The crystal structures and inhibitor complexes of two industrially important ω-aminotransferase enzymes from Pseudomonas aeruginosa and Chromobacterium violaceum have been determined in order to understand the differences in their substrate specificity. The two enzymes share 30% sequence identity and use the same amino acceptor, pyruvate; however, the Pseudomonas enzyme shows activity towards the amino donor β-alanine, whilst the Chromobacterium enzyme does not. Both enzymes show activity towards S-α-methylbenzylamine (MBA), with the Chromobacterium enzyme having a broader substrate range. It appears that the different rigidity of the protein scaffold contributes to the substrate specificity observed for the two ω-­aminotransferases.

We also present the crystal structure of C. violaceum Am:PyAT in complex with the inhibitor gabaculine. In comparison, the crystal structure of the C. violaceum gabaculine complex shows significant structural rearrangements from the structures of both the apo and holo forms of the enzyme. The C. violaceum Am:PyAT–mCPP complex was refined with partial occupancies of 0.7 and 0.6 in subunits A and B, respectively. The loop CV Ala57–Cys61 in chain A of the C. violaceum Am:PyAT–mCPP complex was built in two alternative conformations. The major conformation of this loop in chain A (occupancy of 0.7) folds differently, with the positions of CV Leu59 and CV Trp60 inverted at the bottom of the substrate pocket. The mCPP aromatic ring is rotated by approximately 15° between the two subunits of the C. violaceum Am:PyAT–mCPP complex. The carboxyl group of gabaculine forms a salt bridge with the side chain of CV Arg416 in the C. violaceum enzyme structure. The aromatic ring of mCPP is positioned in a hydrophobic pocket formed by residues CV Trp60, CV Tyr153, CV Ala231, CV Ile262, CV Leu59 and CV His318 from the adjacent subunit. The mCPP complex with the phosphate group bound in the same place is almost as open as the apoenzyme structure. In the inhibitor-bound structure the enzyme is conformationally relaxed in a state between the apoenzyme and holoenzyme structures.

>[2x]MQKQRTTSQWRELDAAHHLHPFTDTASLNQAGARVMTRGEGVYLWDSEGNKIIDGMAGLWCVNVGYGRKDFAEAARRQMEELPFYNTFFKTTHPAVVELSSLLAEVTPAGFDRVFYTNSGSESVDTMIRMVRRYWDVQGKPEKKTLIGRWNGYHGSTIGGASLGGMKYMHEQGDLPIPGMAHIEQPWWYKHGKDMTPDEFGVVAARWLEEKILEIGADKVAAFVGEPIQGAGGVIVPPATYWPEIERICRKYDVLLVADEVICGFGRTGEWFGHQHFGFQPDLFTAAKGLSSGYLPIGAVFVGKRVAEGLIAGGDFNHGFTYSGHPVCAAVAHANVAALRDEGIVQRVKDDIGPYMQKRWRETFSRFEHVDDVRGVGMVQAFTLVKNKAKRELFPDFGEIGTLCRDIFFRNNLIMRACGDHIVSAPPLVMTRAEVDEMLAVAERCLEEFEQTLKARGLA> LNIDMNWLGQLLGSDWEIFPAGGATGDAYYAKHNGQQLFLKRNSSPFLAVLSAEGIVPKLVWTKRMENGDVITAQHWMTGRELKPKDMSGRPVAELLRKIHTSKALLDMLKRLGKEPLNPGALLSQLKQAVFAVQQSSPLIQEGIKYLEEHLHEVHFGEKVVCHCDVNHNNWLLSEDNQLYLIDWDGAMIADPAMDLGPLLYHYVEKPAWESWLSMYGIELTESLRLRMAWYVLSETITFIAWHKAKGNDKEFHDAMEELHILMKRIVD

CcrZ is a recently discovered cell cycle regulator that connects DNA replication initiation with cell division in pneumococci and may have a similar function in related bacteria. The CcrZ structure most closely resembles choline kinases, consisting of a bilobal structure with a cleft between the two lobes for binding ATP and substrate. Instead, CcrZ shows activity on D-ribose and 2-deoxy-D-ribose, indicating adaptation of the choline kinase fold in CcrZ to phosphorylate a novel substrate. We show that integrity of the kinase active site is required for ATPase activity in vitro and for function in vivo.

The structure of CcrZ-AMP-PNP was determined by single-wavelength anomalous diffraction using SelenoMet-CcrZ crystals at a resolution of 2.6 Å. Structural alignment of the CcrZ-AMP-PNP structure with LicA confirmed the conservation of an N-terminal lobe (aa 1–79 in CcrZ) containing the P-loop (22GGATG26 based on alignment with LicA) and other residues important for ATP-binding and kinase activity, and a C-terminal lobe (aa 80–268 in CcrZ) harboring the putative substrate-binding pocket. However, in contrast to LicA, the cleft between the N- and C-terminal lobes is wider in the CcrZ-AMP-PNP structure, which could provide insights into how choline kinase activity may be lost in CcrZ. Inspection of the AMP-PNP in the CcrZ structure revealed that the adenine base is sandwiched between hydrophobic/aromatic residues lining the bilobal cleft (F39 and W77 of the N-terminal lobe, and L173 and I183 of the C-terminal lobe) like the LicA-AMP-MES structure. However, in contrast to the nucleotide-bound LicA structure, the orientation of AMP-PNP is in the opposite orientation in the CcrZ structure. Instead of occupying the active site, the AMP-PNP moiety is rotated such that the sugar and phosphates are facing out of the active site despite the placement of the adenine base in its pocket within the enzyme. In agreement with a non-canonical AMP-PNP engagement in the kinase site of CcrZ, several P-loop residues of CcrZ remain unresolved in the electron density. We propose that our structure captures a state of the enzyme between its apo and substrate-bound forms. Almost all of the bulky side-chains that form the cage surrounding choline in LicA are replaced by smaller residues in the CcrZ structure. Specifically, LicA residues M28, Y197, W251, and Y268 are substituted in CcrZ by A24, G187, F240, and A256, respectively.>[2x]ASSTNLKDILADLIPKEQARIKTFRQQ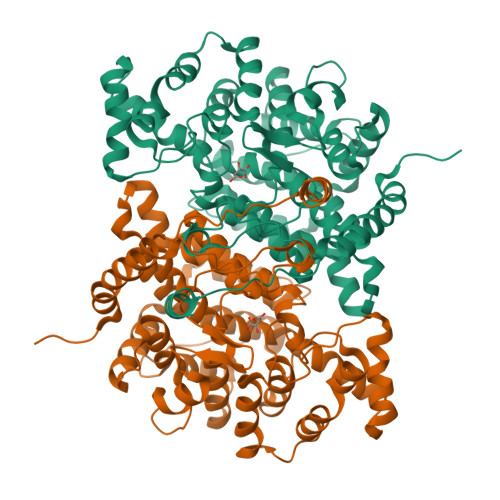HGNTVVGQITVDMMYGGMRGMKGLVYETSVLDPDEGIRFRGYSIPECQKMLPKAKGGEEPLPEGLFWLLVTGQIPTEEQVSWLSKEWAKRAALPSHVVTMLDNFPTNLHPMSQLSAAITALNSESNFARAYAEGIHRTKYWELIYEDCMDLIAKLPCVAAKIYRNLYREGSSIGAIDSKLDWSHNFTNMLGYTDAQFTELMRLYLTIHSDHEGGNVSAHTSHLVGSALSDPYLSFAAAMNGLAGPLHGLANQEVLVWLTQLQKEVGKDVSDEKLRDYIWNTLNSGRVVPGYGHAVLRKTDPRYTCQREFALKHLPHDPMFKLVAQLYKIVPNVLLEQGKAKNPWPNVDAHSGVLLQYYGMTEMNYYTVLFGVSRALGVLAQLIWSRALGFPLERPKSMSTDGLIKLVDSK> ALSR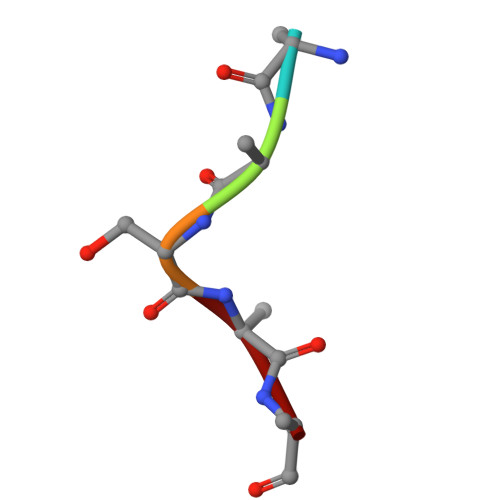Q>MANCERTFIAIKPDGVQRGLVGEIIKRFEQKGFRLV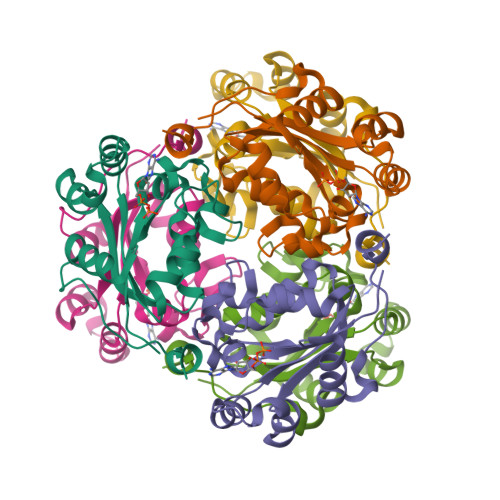GLKFMQASEDLLKEHYVDLKDRPFFAGLVKYMHSGPVVAMVWEGLNVVKTGRVMLGETNPADSKPGTIRGDFCIQVGRNIIHGGDSVESAEKEIGLWFHPEELVDYTSCAQNWIYE[3x]> MNAFRLTVEVNGVTHATDVEPRRLLADFLRDDLHLRGTRVG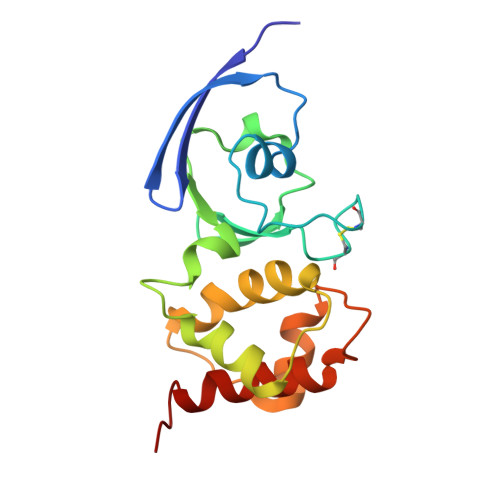CEHGVCGSCTVILDGQPVRSCTVLAVQANNSRIETVESLQKDGQLHPLQRSFSKCHALQCGFCTSGFLMTLKPLYDDEDVTLDATSAREAISGNLCRCTGYQQIVEATVDAFHCRDHND> MEFFGESWKKHLSGEFGKPYFIKLMGFVAEERKHYTVYPPPHQVFTWTQMCDIKDVKVVILGQDPYHGPNQAHGLCFSVQRPVPPPPSLENIYKELSTDIEDFVHPGHGDLSGWAKQGVLLLNAVLTVRAHQANSHKERGWEQFTDAVVSWLNQNSNGLVFLLWGSYAQKKGSAIDRKRHHVLQTAHPSPLSVYRGFFGCRHFSKTNELLQKSG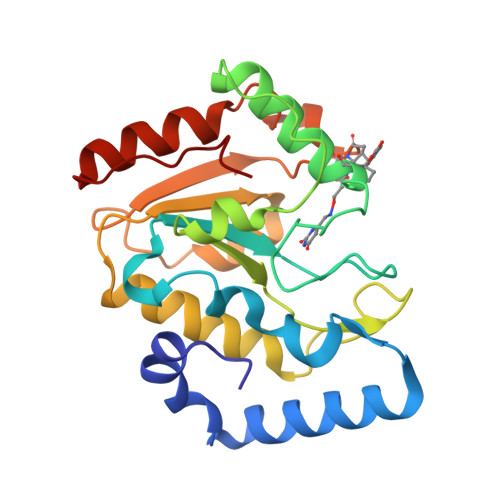KKPIDWKEL The sigma-1 receptor (σ1R) is an endoplasmic reticulum (ER)-localized, non-opioid transmembrane receptor implicated in many pathological conditions, including neurodegenerative disorders and cancer. So far, all reported σ1R structures are homotrimers, with the ligand binding site located inside the β-barrel domain of each σ1R monomer. The ligand binding site is located in the lumen of the β-barrel domain (β1-β10), whose opening is covered by two membrane-adjacent helices (α4/α5) at the carboxy-terminus. Here, we present crystal structures of σ1R from Xenopus laevis (xlσ1R) bound to two endogenous neurosteroid ligands, progesterone (a putative antagonist) and dehydroepiandrosterone sulfate (DHEAS) (a putative agonist), at 2.15-3.09  Å resolutions.

Interestingly, in addition to the α4/α5-entrance and the hinge-entrance, the simulations revealed a third potential entrance located between the α4 helix (near S177 and F181) and the β4/β5 loop near R116 (termed side-entrance). Therefore, we solved structures for ~30 randomly selected xlσ1R crystals and eventually succeeded in capturing a xlσ1R structure at 2.81  Å with the side-entrance open (termed xlσ1Rside-open). The xlσ1Rside-open structure was solved in the C2 space group, with six protomers (two trimers) in each asymmetric unit. Among them, two protomers (A and B) are in a side-closed conformation similar to xlσ1Runknown-lig/xlσ1Rprog-co. The other four protomers (C, D, E and F) adopt a side-open conformation with an open side-entrance, similar to that observed in the simulations. Solvent accessibility analysis of the side-open protomer (e.g. protomer C) showed a clear opening surrounded by residues 114-118 (β4/β5 loop) and 177-181 (α4). Comparison of the side-open and the side-closed conformations revealed that a local conformational rearrangement of Y117 and W118 on the β4/β5 loop leads to open or close of the side-entrance. In xlσ1Rside-open, W118 of a side-open protomer (e.g. protomer C) is 4–5  Å away from Q191 and F193 (α4/α5 loop) of protomer A. Moreover, the side-entrance gives solvent immediate access to residues such as S114 (β4/β5 loop), Y117 (β4/β5 loop), D123 (β5) and H151 (β8), which are the coordinating residues for water molecules in the distal β-barrel lumen in the xlσ1Rprog-co structure. This data suggests that the side-entrance may be a potential water entrance that allows water to reach the distal region of the β-barrel lumen.

>GGGGRSVDTMALWLGLRAVLVVAGLAVLLQLIRGWLSSKSYVFNREEIARLAKEHSGLDYEVAFSKIIVELRKKHPGHILQDEDLQWVFVNAGGWMGSMCLLHASLTEYVLLFGTAVDTGGHSGRYWAEISDTILSGTFRQWKEGTTKSEIFYPGDTIVHEVGEATSVQWSSGTWMVEYGRGFIPSTLAFALADTIFSTQDFLTLFYTVKVYSKALLLEASTHLSQLGFFAAA[6x]>[2x]MTTGLSTAGAQDIGRSSVRPYLEECTRRFQEMFDRHVVTRPTKVELTDAELREVIDDCNAAVAPLGKTVSDERWISYVGVVLWSQSPRHIKDMEAFKAVCVLNCVTFVWDDMDPALHDFGLFLPQLRKICEKYYGPEDAEVAYEAARAFVTSDHMFRDSPIKAALCTTSPEQYFRFRVTDIGVDFWMKMSYPIYRHPEFTEHAKTSLAARMTTRGLTIVNDFYSYDREVSLGQITNCFRLCDVSDETAFKEFFQARLDDMIEDIECIKAFDQLTQDVFLDLIYGNFVWTTSNKRYKTAVNDVNSRIQAAALEHHHHHH

To elucidate the dynamic interactions of TPSs with their substrates during catalysis, we investigated the bacterial diterpene synthase CotB2 as a model system. CotB2 adopts an α-helical bundle fold that is conserved among class I TPSs (PDB-ID 4OMG17). The CotB2 protein sequence exhibits a modified aspartate-rich DDXD motif12 deviating from the conventional DDXXD motif and the NSE triad NDXXSXX(R,K)(E,D) as found in bacteria and fungi, that is altered to a DTE triad in plants. Upon substrate and Mg2+ binding, TPSs undergo a discrete conformational change from an open, catalytically inactive one to a catalytically active closed conformation.

In this study, we intended to probe the structural dynamics of the CotB2 reaction using X-ray crystallography of the catalytically relevant protein states in the presence of a substrate-analogue. Remarkably, we could capture the closed conformation of CotB2 by co-crystallisation with the substrate-analogue 2-fluoro GGDP (FGGDP) and determined the crystal structure at 1.8 Å (CotB2wt•Mg2+3•F-Dola (2-fluoro-3,7,18-dolabellatriene); Figs. 1c, d, 2a, Supplementary Table 2). FGGDP is functionalised with a fluorine atom at the C2 position of its hydrophobic tail that interferes with the propagation of the generated carbocation(s). Upon binding of FGGDP the 12 C-terminal residues are structured to fold over the active site, resulting in the fully active and closed conformation. Surprisingly, we did not observe the entire FGGDP molecule. Instead, we detected clearly resolved electron density for a single diphosphate moiety and for a ring-like structure positioned in the active site that we interpret as the reaction intermediate 2-fluoro-3,7,18-dolabellatriene (F-Dola). Most likely the fluorinated substrate alters propagation of the carbocation and hence we do not observe the native product. Additionally, active site residues R227 and R294 make contact with the oxygen atoms of the diphosphate moiety to compensate its negative charge. The closure by the C-terminus is initiated by formation of a salt-bridge between D111 and R294. Additionally, Y295 establishes hydrogen bonds to the diphosphate moiety derived from FGGDP as well as to N220 of the NSE motif.>[3x]MQPMTARFDLFVVGSGFFGLTIAERVATQLDKRVLVLERRPHIGGNAYSEAEPQTGIEVHKYGAHLFHTSNKRVWDYVRQFTDFTDYRHRVFAMHNGQAYQFPMGLGLVSQFFGKYFTPEQARQL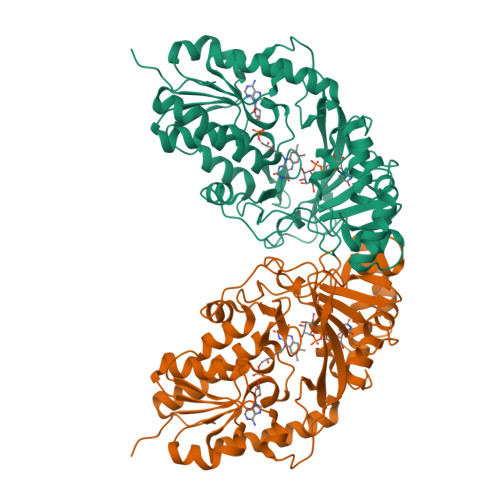IAEQAAEIDTADAQNLEEKAISLIGRPLYEAFVKGYTAKQWQTDPKELPAANITRLPVRYTFDNRYFSDTYEGLPTDGYTAWLQNMAADHRIEVRLNTDWFDVRGQLRPGSPAAPVVYTGPLDRYFDYAEGRLGWRTLDFEVEVLPIGDFQGTAVMNYNDLDVPYTRIHEFRHFHPERDYRTDKTVIMREYSRFAEDDDEPYYPINTEADRALLATYRARAKSETASSKVLFGGRLGTYQYLDMHMAIASALNMYDNVLAPHLRDGVPLLQDGA> G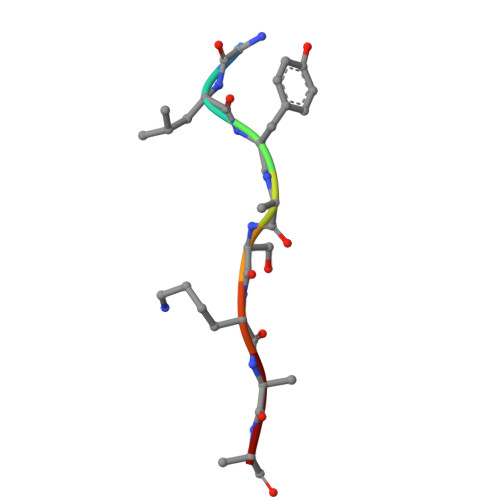LYASKLA> MENTENSVDSKSIKNLEPKIIHGSESMDSGISLDNSYKMDYPEMGLCIIINNKNFHKSTGMTSRSGTDVDAANLRETFRNLKYEVRNK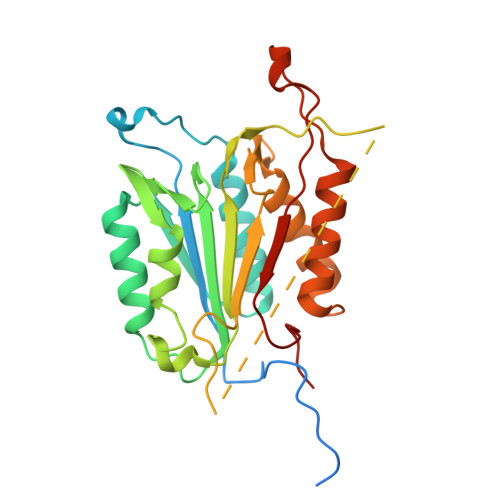NDLTREEIVELMRDVSKEDHSKRSSFVCVLLSHGEEGIIFGTNGPVDLKKITNFFRGDRCRSLTGKPKLFIIQACRGTELDCGIETDSGVDDDMACHKIPVEADFLYAYSTAPGYYSWRNSKDGSWFIQSLCAMLKQYADKLEFMHILTRVNRKVATEFESFSFDATFHAKKQIPCICSMLTKELYFYHL>MGSSHHHHHHENLYFQGTSKPESPQRCLGRPAPADLPLGLDPFCYRQFDDPAYGGSRISGVTKEEFLEKVNELVTRDAGIEFFQGYAPFCRHLYIPNFVGALPGSLPITADNEHLLRSGYIARRPNELPVLTRWFPMSYAKDALMPAAFLDL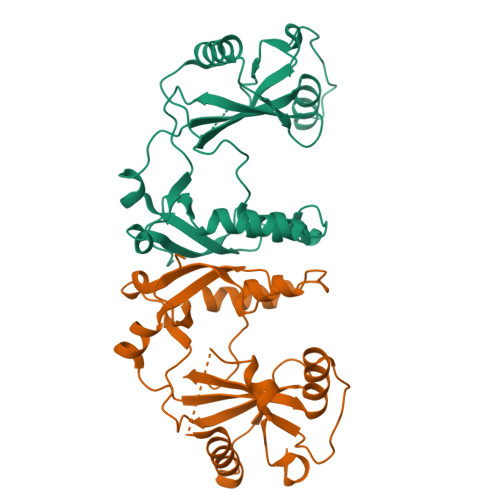ILYSREQIAKETAAESNTAVVIDPNAPAWSIIAVKAQNEKYSLPMAPITMLRNTLIEEGGSGVALDREAYKASVAYWKTHAIVMDKESSLE[2x]>GAMGSKPDTHRADERRFLDERGSSGPLAPNGLNPATIMEKAVRERIVESYFWKEQCFGVNEADIVDRVVEHVRFVGGVTGVTQKPSPFLCLAFKLLQLAPGDDILKEYLYFGGEKFKYLRALAAFYIRLTRPDKEVYTLLEPFLEDRRKLRRKGKNGTSLTYMDEFIDDLLTKDRVCSTSLWKMRRRDILEDLDLLEPRVSPLGSLEDILEEEEQAAKNEDGE[3x];>[3x]GAMGTTDDVDPEAEYAAWKLRELRRLRRERDAIEARERELAELERRR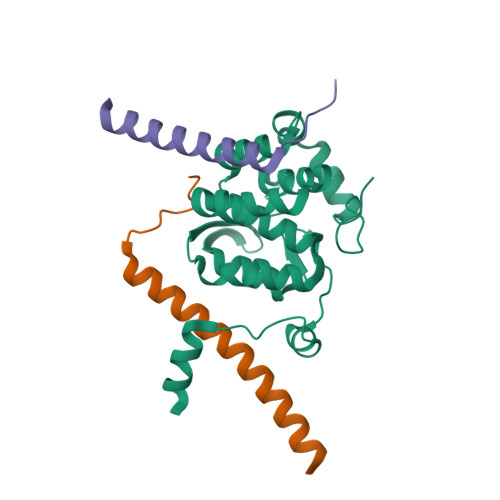NLTEEERRAEDEAHLAKQKAEKESRGKMGYLQKYFHR;>GAGEVKKATAEEVHARIEFLWQREQEKKKEQVVSLK[3x]>[2x]QNMEGNGPAAVHYQPASPPRDACVYSSCYSEENVWKLCEYIKNHDQYPLEECYAVFISNERKMIPIWKQQARPGDGPVIWDYHVVLLHVSSGGQSFIY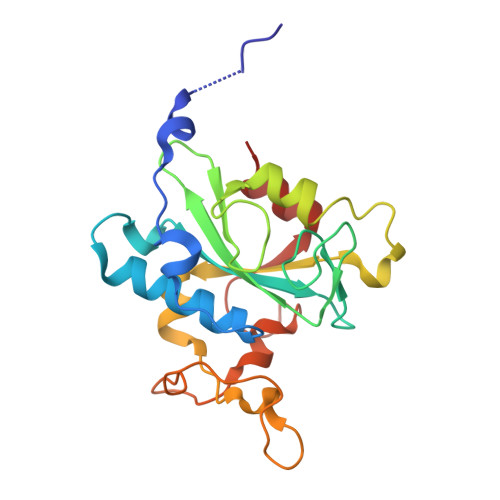DLDTVLPFPCLFDTYVEDAIKSDDDIHPQFRRKFRVICADSYLKNFASDRSHMKDSSGNWREPPPPYPCIETGDSKMNLNDFISMDPKVGWGAVYTLSEFTHRFGS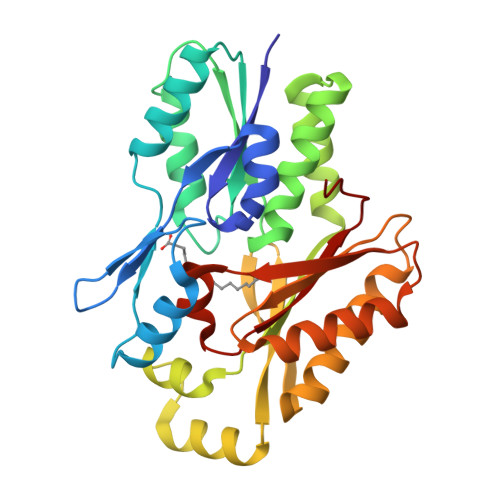>HMKIAVMTDSTSYLSQDLIDKYNIQIAPLSVTFDDGKNFTESNEIAIEEFYNKMASSQTIPTTSQPAIGEWITKYEMLRDQGYTDIIVICLSSGISGSYQSSYQAGEMVEGVNVHAFDSKLIAMIEGCYVLRAIEMVEEGYEPQQIIDDLTNMREHTGLYLIVDDLKNLQKSGRITGAQAWVGTLLKMKPVLKFEDGKIIPEEKVRTKKRAIQTLEKKVLDIVKDFEEVTLFVINGDHFEDGQALYKKLQDDCPSAYQVAYSEFGPVVAAHLGSGGLGLGYVGRKIRLT[2x]(2R,3R,4S,5S,6R)-3,4-dihydroxy-5-[(E)-({3-hydroxy-2-methyl-5-[(phosphonooxy)methyl]pyridin-4-yl}methylidene)amino]-6-methyloxan-2-yl 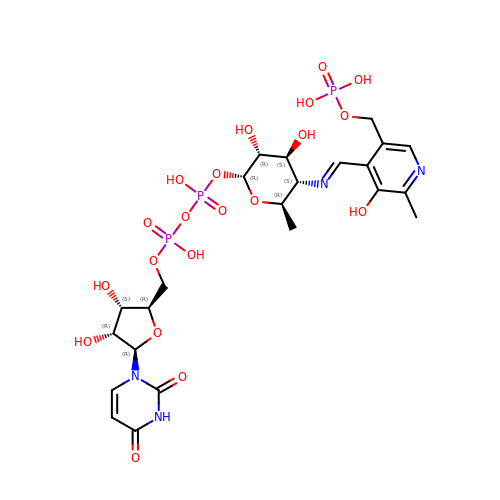[(2R,3S,4R,5R)-5-(2,4-dioxo-3,4-dihydropyrimidin-1(2H)-yl)-3,4-dihydroxyoxolan-2-yl]methyl dihydrogen diphosphate (non-preferred name) | C23 H33 N4 O20 P3 | YCGRRMXEGFNOLB-XUIBUIKDSA-N> MHHHHHHTTTATGTTGSLAADPVTVLGLGDMGSAI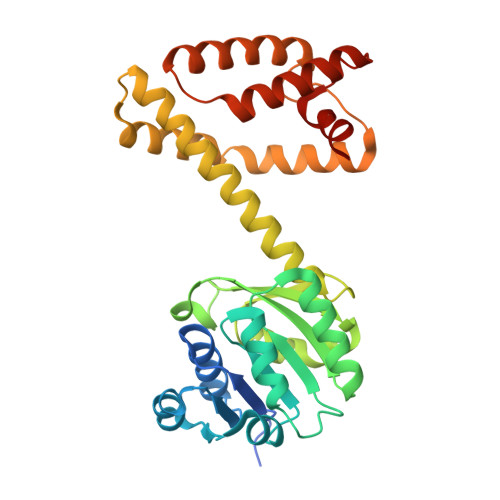ARAFVERGHRTTVWNRTASKCRPLVEAGASAAATPDEAVEASRFVVVCLLDSAAVDEVLGSVTSSLAGKVLVNLTSGSPSQARSNERWARERGAEYLDGKIMGDPPDVGTSNVSLSFSGSRSAFDAHEPILRELGGVAYHGEDAGLAAVEFLAQVAMGYELLIGFLHTLSVVHAEGVEVEAFAERVAGSVAAYPPLLTMMGKAIGSGEYGPDLGSLRVQAALMDDLISHRESLGVEAVRMREVKELMDQRIADGHGGQGFSSLFELLTKR> CSVHAECRDYATGFCCRCVANYTGNGRQCVAEGSPQRVNGKVKGRIFVGSSQVPVVFENTDLHSYVVMNHGRSYTAISTIPETVGYSLLPLAPIGGIIGWMFAVEQDGFKNGFSITGGEFTRQAEVTFLGHPGKLVLKQQFSGIDEHGHLTISTELEGRVPQIPYGASVHIEPYTELYHYSSSVITSSSTREYTVMEPDQD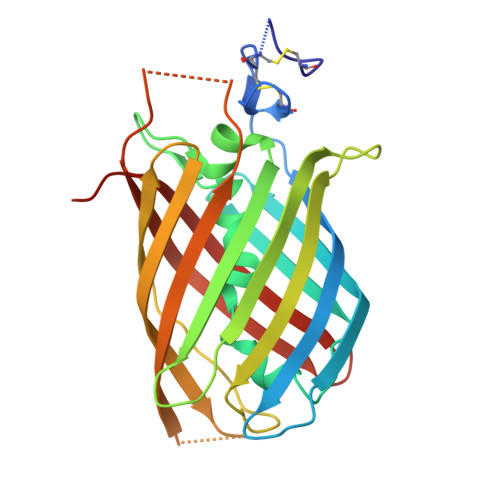GAAPSHTHIYQWRQTITFQECAHDDARPALPSTQQLSVDSVFVLYNKEERILRYALSNSIGPVR>MAVLGLQGVRGGVGTTTITAALAWSLQMLGENVLVVDACPDNLLRLSFNVDFTHRQGWARAMLDGQDWRDAGLRYTSQLDLLPFGQLSIEEQENPQHWQTRLSDICSGLQQLKASGRYQWILIDLPRDASQITHQLLSLCDHSLAIVNVDANCHIRLHQQALPDGAHILINNFRIGSQVQDDIYQLWLQSQRRLLPMLIHRDEAMAECLAAKQPVGEYRSDALAAEEILTLANWCLLNYSGLKTPVGSKSAAALEHHHHHH[3x];>[2x]MNNNEPDTLPDPAIGYIFQNDIVALKQAFSLPDIDYADISQREQLAAALKRWPLLAE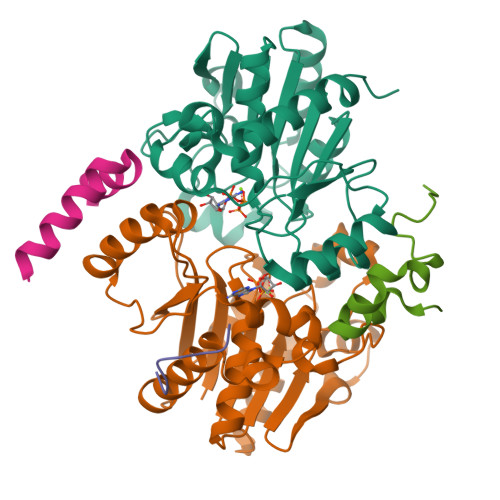FAQQK4-{4-[3-(2-bromo-5-fluorophenoxy)propyl]phenyl}-N-(2-chlorobenzyl)-N-cyclopropyl-1,2,5,6-tetrahydropyridine-3-carboxamide | C31 H31 Br Cl F N2 O2 | 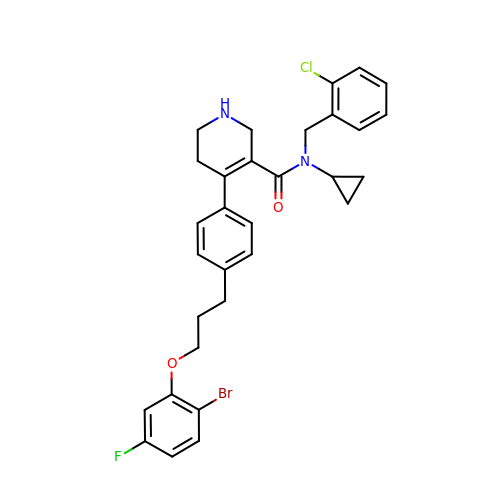GNQKDXQPKKYVIX-UHFFFAOYSA-N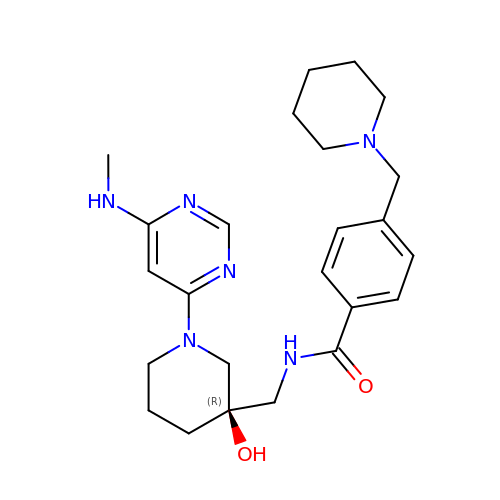N-[[(3R)-3-Hydroxy-1-[6-(methylamino)pyrimidin-4-yl]piperidin-3-yl]methyl]-4-(piperidin-1-ylmethyl)benzamide | C24 H34 N6 O2 | OUFLYLBALJIUPJ-XMMPIXPASA-N> GSDELYRQSLEIISRYLREQATGAKDTKPMGRSGATSRKA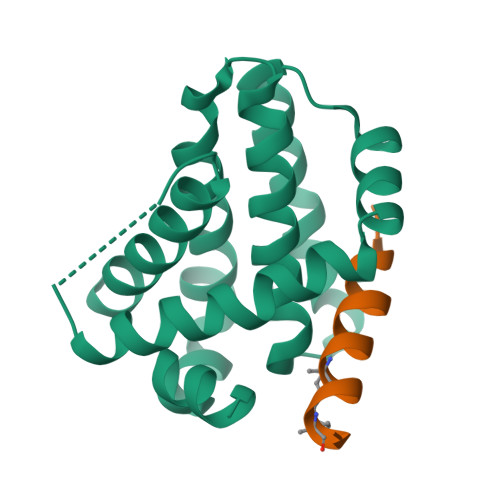LETLRRVGDGVQRNHETAFQGMLRKLDIKNEDDVKSLSRVMIHVFSDGVTNWGRIVTLISFGAFVAKHLKTINQESCIEPLAESITDVLVRTKRDWLVKQRGWDGFVEFFHVEDLEGG;> KALETLRRVGDGVLRNHLTAF> KTAAPVQET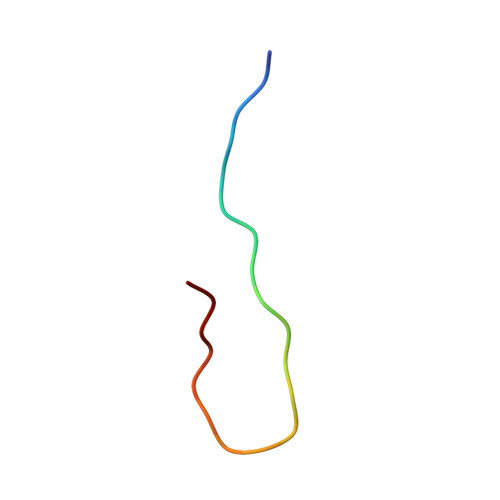LHGSQPVTQEDG> MTAAEHGLHAPAYAWSHNGPFETFDHASIRRGYQVYREVCAACHSLDRVAWRTLVGVSHTNEEVRNMAEEFEYDDEPDEQGNPKKRPGKLSDYIPGPYPNEQAARAANQGALPPDLSLIVKARHGGCDYIFSLLTGYPDEPPAGVALPPGSNYNPYF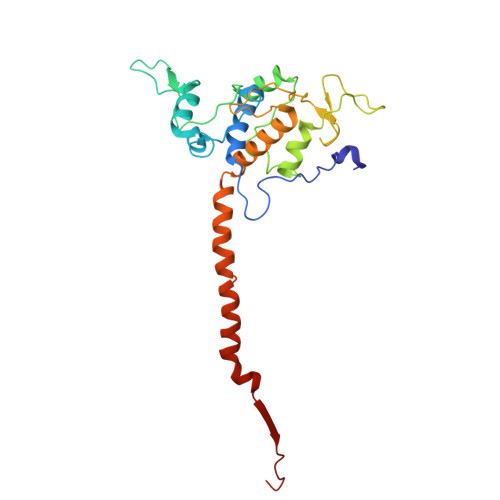PGGSIAMARVLFDDMVEYEDGTPATTSQMAKDVTTFLNWCAEPEHDERKRLGLKTVIILSSLYLLSIWVKKFKWAGIKTRKFVFNPPKPRK VARP is a Rab32/38 effector that also binds to the endosomal/lysosomal R-SNARE VAMP7. VARP binding regulates VAMP7 participation in SNARE complex formation and can therefore influence VAMP7-mediated membrane fusion events. Rab32 is an endosomal Rab GTPase, thought to have been present in the last eukaryotic common ancestor, with Rab38 arising in vertebrates as an evolutionary gene duplication of Rab32 (Klöpper et al., 2012). VARP has been shown to interact with Rab32/38 via its first ankyrin repeat-containing domain (Tamura et al., 2009, 2011; Wang et al., 2008).

We determined the crystal structure of the complex between the first ankyrin repeat domain of VARP with the GTP hydrolysis-deficient forms of Rab32 and Rab38. Many small GTPase:effector complexes are believed to form dimers, which increases both the apparent affinity and specificity of the recruitment of effectors to membrane-anchored GTPases (Lee et al., 2009; Panic et al., 2003). In the crystal, all VARP:Rab32 heterodimers form identical homodimers, resulting in the heterotetramers shown in Figures 1C and 1D. Further evidence comes from size exclusion chromatography with multiangle light scattering (data not shown), as well as the observation that, in crystals, VARP ANKRD1:SeMet-Rab32Q85L and VARP ANKRD1:Rab38Q69L contain the same “cross-dimer of heterodimers” across multiple crystal forms, as compared to the wtVARP:Rab32Q85L complex. The majority of the heterodimer/heterodimer interface arises from the VARP molecules contacting the other Rab32 molecule in the tetramer through residues from Switch-I and Switch-II that are different from those involved in the VARP:Rab32 heterodimer formation. This second VARP:Rab32 interface buries 1,460 Å2 of solvent accessible surface area, making the total solvent accessible buried surface area on tetramer formation around 6,400Å2, which suggests that the tetramer should be stable. Existence of a dimer of heterodimers in solution is supported by analytical gel filtration, which is consistent with the existence of a concentration-dependent equilibrium of a 2:2 tetramer and a 1:1 heterotetramer in solution.

>[3x]GPLGSMAGGGAGDPGLGAAAAPAPETREHLFKVLVIGELGVGKTSIIKRYVHQLFSQHYRATIGVDFALKVLNWDSRTLVRLQLWDIAGLERFGNMTRVYYKEAMGAFVVFDISRSSTFEAVLKWKSDLDSKVHLPNGSPIPAVLLANKCDQNKDSSMSPSQMDQFCKEHGFAGWFETSAKDNINIEEAARFLVEKMLVNHQSFPNEENDVDKIKLDQETLRAENKSQCC;>[3x]GPLGSMDPSVVTPFSRDDRGHTPLHVAAVCGQASLIDLLVSKGAMVNATDYHGATPLHLACQKGYQSVTLLLLHYKASAEVQDNNGNTPLHLACTYGHEDCVKALVYYDVESCRLDIGNEKGDTPLHIAARWGYQGVIETLLQNGASTEIQNRLKETPLKCALNSKILSVMEAYHLSFERRQKSSEAPVQSPQRSVDHHHHHH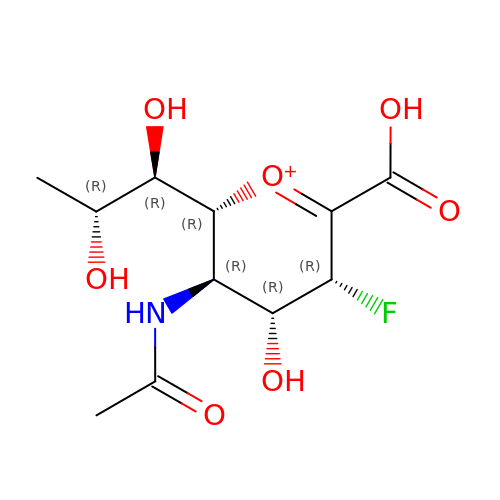(2~{R},3~{R},4~{R},5~{R})-3-acetamido-2-[(1~{R},2~{R})-1,2-bis(oxidanyl)propyl]-5-fluoranyl-4-oxidanyl-2,3,4,5-tetrahydropyran-1-ium-6-carboxylic acid | C11 H17 F N O7 | DTEWGJXDNGDFKL-IHBVAVKPSA-O Specifically, the β-­glycosidic bond of 6′-P-β-glucoside is cleaved by 6-P-β-glucosidase (6PβGlu; EC 3.2.1.86), releasing 6-P-β-glucose (BG6; glycon), an important cellular precursor, and the remaining portion of the given substrate (aglycon). Here, the high-resolution crystal structures of GH1 6-P-β-glucosidases from Lactobacillus plantarum (LpPbg1) and Streptococcus mutans (SmBgl) and their complexes with ligands are reported. 6PβGlu is a single-domain protein that adopts a (β/α)8-barrel (TIM-barrel) structure, which is a typical fold of GH1-family members. The GH1-family enzymes utilize a double-displacement mechanism of catalysis with retention of configuration at the anomeric C atom of the glycon moiety.

For a mutated variant of the S. mutans enzyme (E375Q), the structure of a 6′-P-salicin complex has also been determined. The E375Q SmBgl–PSC crystals belonged to the tetragonal system, with one protein molecule present in the asymmetric unit of the P41212 unit cell. In the E375 QSmBgl–PSC structure the aromatic moiety of PSC occupies the aglycon site. Substrate-bound and product-bound complexes of SmBgl contain a phosphoryl group attached to the glucose ring occupying the phosphate-dedicated cavity. An analogous set of interactions links the anion (or a phosphoryl group) in SmBgl (E375Q SmBgl–PSC), with the exception of Ser432, which is substituted by Gly432, resulting in the elimination of one hydrogen bond. Interestingly, the active-site E375Q SmBgl mutant also showed some residual catalytic activity (0.8% of the wild-type enzyme activity detected for gentiobiose).

> SNAMSKLPENFLWGGAVAAHQLEGGWQEGGKGISVADVMTAGRHGVAREITAGVLEGKYYPNHEAIDFYHHYKEDVKLFAEMGFKCFRTSIAWTRIFPKGDEAEPNEAGLQFYDDLFDECLKYGIEPVVTLSHFELPYHLVTEYGGFTNRKVIDFFVHFAEVCFRRYKDKVKYWMTFNEINNQANYQEDFAPFTNSGIVYKEGDDREAIMYQAAHYELVASARAVKIGHAINPNLNIGCMVAMCPIYPATCNPKDILMAQKAMQKRYYFADVHVHGFYPEHIFKYWERKAIKVDFTERDKKDLFEGTVDYIGFSYYMSFVIDAHRENNPYYDYLETEDLVKNPYVKASDWDWQIDPQGLRYALNWFTDMYHLPLFIVQNGFGAIDQVEADGMVHDDYRIDYLGAHIKEMIKAVDEDGVELMGYTPWGCIDLVSAGTGEMRKRYGFIYVDKDDEGKGTLKRSPKLSFNWYKEVIASNGDDI>TSCNPSDMSHGYVTVKPRVRLHFVELGSGPAVCLCHGFPESWYSWRYQIPALAQAGYRVLAMDMKGYGESSAPPEIEEYCMEVLCKEMVTFLDKLGLSQAVFIGHDWGGMLVWYMALFYPERVRAVASLNTPFIPANPNMSPLESIKANPVFDYQLYFQEPGVAEAELEQNLSRTFKSLFRASDESVLSMHKVCEAGGLFVNSPEEPSLSRMVTEEEIQFYVQQFKKS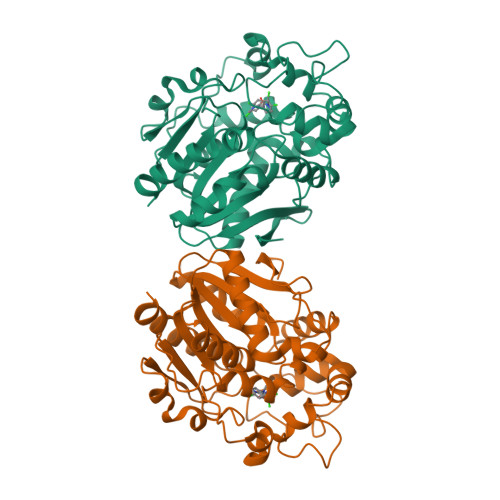GFRGPLNWYRNMERNWKWACKSLGRKILIPALMVTAEKDFVLVPQMSQHMEDWIPHLKRGHIEDCGHWTQMDKPTEVNQILIKWLDSDARNPPVVSKM[2x]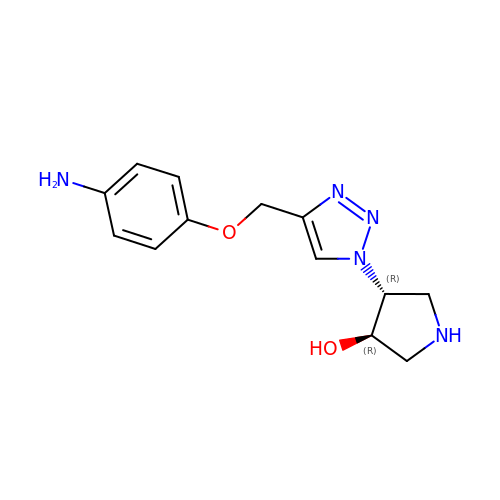(3~{R},4~{R})-4-[4-[(4-azanylphenoxy)methyl]-1,2,3-triazol-1-yl]pyrrolidin-3-ol | C13 H17 N5 O2 | WHSXTRCFXOPSRO-CHWSQXEVSA-N> XEAMPPTLPHRD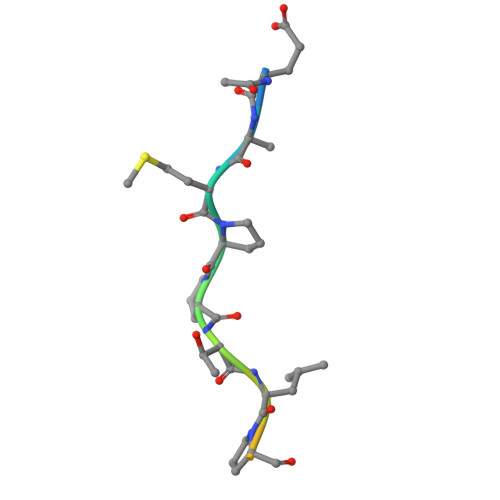WKD> MERTLDRVGVFAATHAAVAASDPLQARALVLQLPGLNRNKDVPGIVGLLREFLPVRGLPSGWGFVEAAAAMRDIGFFLGSLKRHGHEPAEVVPGLEPVLLDLARATNLPPRET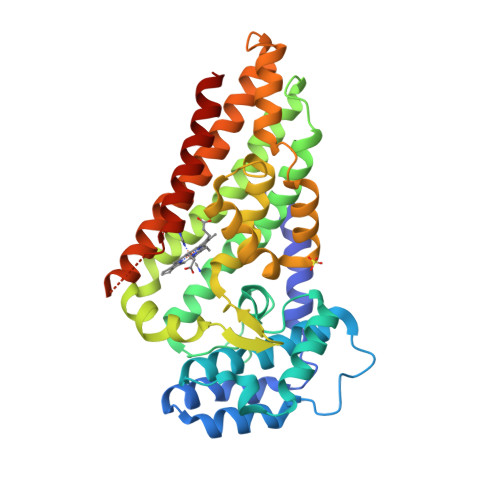LLHVTVWNPTAADAQRSYTGLPDEAHLLESVRISMAALEAAIALTVELFDVSLRSPEFAQRSDELEAYLQKMVESIVYAYRFISPQVFYDELRPFYEPIRVGGQSYLGPGAVEMPLFVLEHVLWGSQSDDQTYREFKETYLPYVLPAYRAVYARFSGEPALIDRALDEARAVGTRDEHVRAGLTALERVFKVLLRFRAPHLKLAERAYEVGQSGPEIGSGGYAPSMLGELLTLTYAARSRVRAALDES> GSHMGVSYEEFQVLVRRVDRMEHSIGSIVSKIDAVIV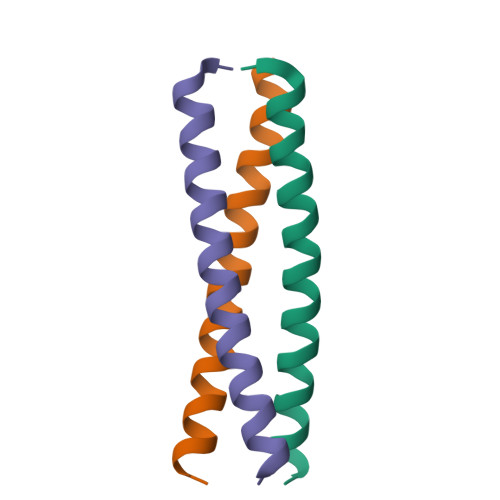KLEIMER> RGGSSTDQPVANPYNTKE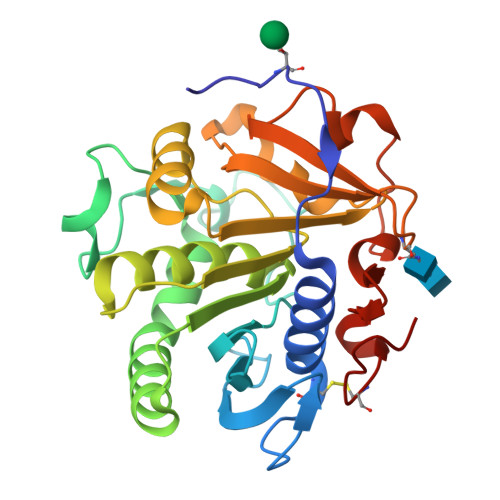ISLAAGLVQQTYCDSTENGLKIGDSELLYTMGEGYARQRVNIYHSPSLGIAVAIEGTNLFSLNSDLHDAKFWQEDPNERYIQYYPKGTKLMHGFQQAYNDLMDDIFTAVKKYKKEKNEKRVTVIGHSLGAAMGLLCAMDIELRMDGGLYKTYLFGLPRLGNPTFASFVDQKIGDKFHSIINGRDWVPTVPPRALGYQHPSDYVWIYPGNSTSAKLYPGQENVHGILTVAREFNFDDHQGIYFHTQIGAVMGECPAQVGAH>MVLYFIGLGLYDERDITVKGLEIAKRCDYVFAEFYTSLMAGTTLGRIQKLIGKEIRVLSREDVELN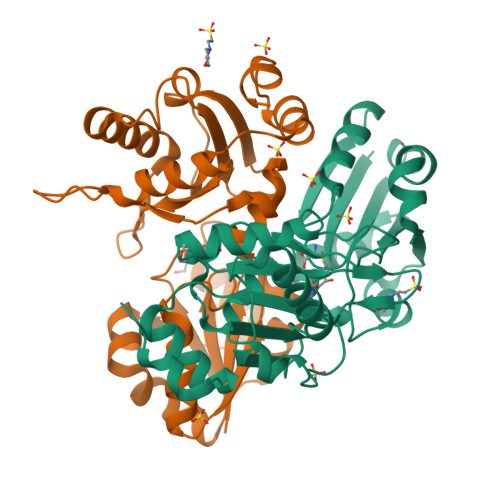FENIVLPLAKENDVAFLTPGDPLVATTHAELRIRAKRAGVESYVIHAPSIYSAVGITGLHIYKFGKSATVAYPEGNWFPTSYYDVIKENAERGLHTLLFLDIKAEKRMYMTANEAMELLLKVEDMKKGGVFTDDTLVVVLARAGSLNPTIRAGYVKDLIREDFGDPPHILIVPGKLHIVEAEYLVEIAGAPREILRVNV[2x]> XLAAHLAQA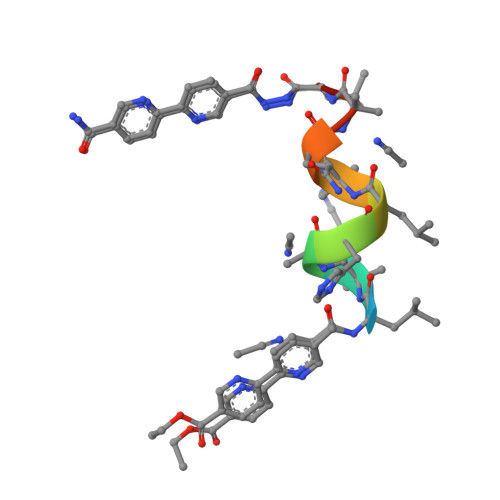LX>[2x]IIGGTECRPHARPYMAYLEIVTPENHLSACSGFLIRRNFVM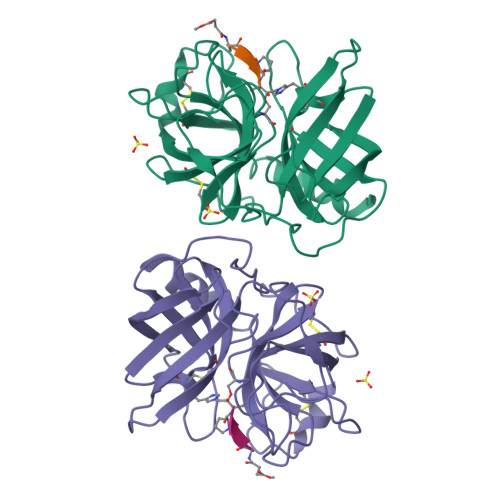TAAHCAGRSITVLLGAHNKKVKEDTWQKLEVEKQFPHPKYDDRLVLNDIMLLKLKEKANLTLGVGTLPISAKSNSIPPGRVCRAVGWGRTNVNEPPSDTLQEVKMRILDPQACKHFEDFHQEPQLCVGNPKKIRNVYKGDSGGPLLCAGIAQGIASYVLRNAKPPSVFTRISHYRPWINKILREN>GSHMASMSKDEVKREAKDTDGNPEIKGERRRLHSEIQSGSLANNIKKSTVIVKN[2x];>[2x]PTHIAICLYYKLGETPLPLVIETGKDAKALQI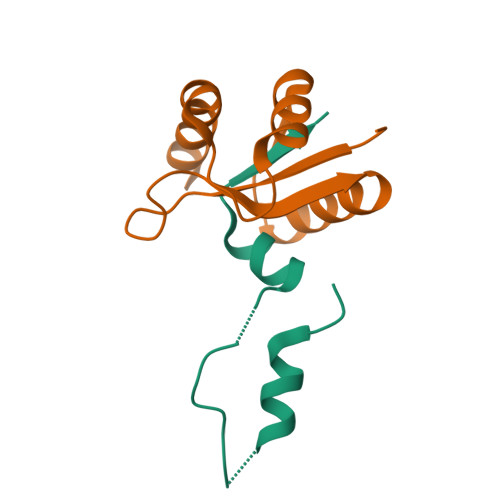IKLAELYDIPVIEDIPLARSLYKNIHKGQYITEDFFEPVAQLIRIAIDLDY> MSHHHHHHSATLNIEDEYRLHETSKEPDVPLGSTWLSDFPQAWAETGGMGLAVRQAPLIIPLKATSTPVSIKQYPMSQEARLGIKPHIQRLLDQGILVPCQSPWNTPLLPVKKPGTNDYRPVQDLREV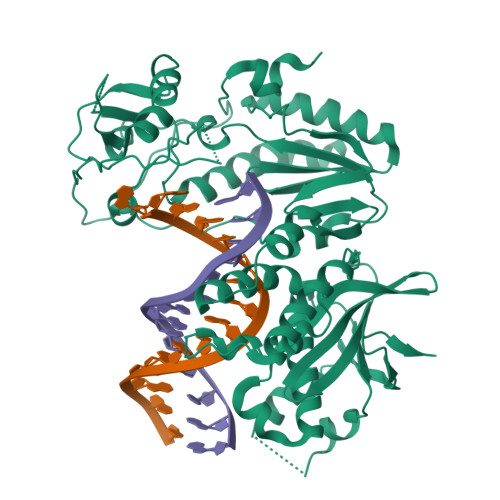NKRVEDIHPTVPNPYNLLSGLPPSHQWYTVLDLKDAFFCLRLHPTSQPLFAFEWRDPEMGISGQLTWTRLPQGFKNSPTLFDEALHRDLADFRIQHPDLILLQYVDDLLLAATSEQDCQRGTRALLQTLGNLGYRASAKKAQICQKQVKYLGYLLKEGQRWLTEARKETVMGQPTPKTPRQLREFLGTAGFCRLWIPGFAEMAAPLYPLTKTGTLFNWGPDQQKAYQEIKQALLTAPALGLPDLTKPFELFVDEKQGYAKGVLTQKLGPWRRPVAYLSKKLDPVAAGWPPCLRMVAAIAVLTKDAGKLTMGQPLVILAPHAVEALVKQPPDRWLSNARMTHYQAMLLDTDRVQFGPVVALNPATLLPLPEKEAPHDCLEILAETHGTRPDLTDQPIPDADYTWYTDGSSFLQEGQRRAGAAVTTETEVIWARALPAGTSAQRAELIALTQALKMAEGKKLNVYTNSRYAFATAHVHGEIYRRRGLLTSEGREIKNKNEILALLKALFLPKRLSIIHCPGHQKGNSAEARGNRMADQAAREAAMKAVLETSTLL>[2x]MAGVLPAHGTQHGIRLPLRSGLGGAPLGLRLPRETDEEPEEPGRRGSFVEMVDNLRGKSGQGYYVEMTVGSPPQTLNILVDTGSSNFAVGAAPHP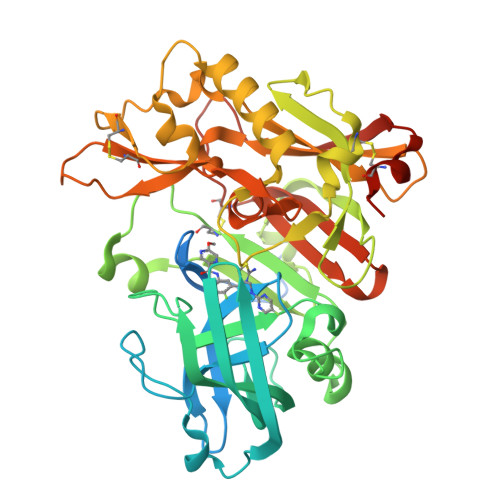FLHRYYQRQLSSTYRDLRKGVYVPYTQGKWEGELGTDLVSIPHGPNVTVRANIAAITESDKFFINGSNWEGILGLAYAEIARPDDSLEPFFDSLVKQTHVPNLFSLQLCGAGFPLNQSEVLASVGGSMIIGGIDHSLYTGSLWYTPIRREWYYEVIIVRVEINGQDLKMDCKEYNYDKSIVDSGTTNLRLPKKVFEAAVKSIKAASSTEKFPDGFWLGEQLVCWQAGTTPWNIFPVISLYLMGEVTNQSFRITILPQQYLRPVEDVATSQDDCYKFAISQSSTGTVMGAVIMEGFYVVFDRARKRIGFAVSACHVHDEFRTAAVEGPFVTLDMEDCGYNIPQTDEST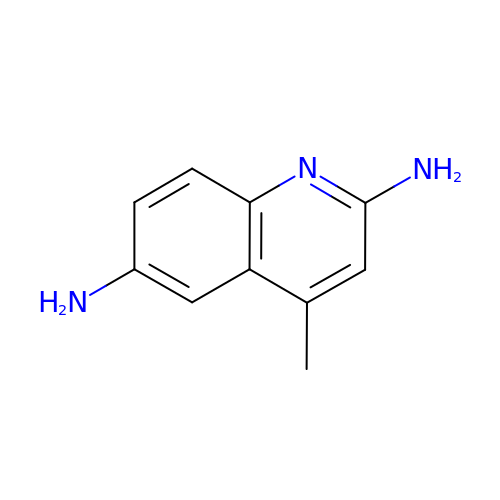4-methylquinoline-2,6-diamine | C10 H11 N3 | RTLBVOMPQYBAQP-UHFFFAOYSA-N> GGUUUCAACAUCCCCG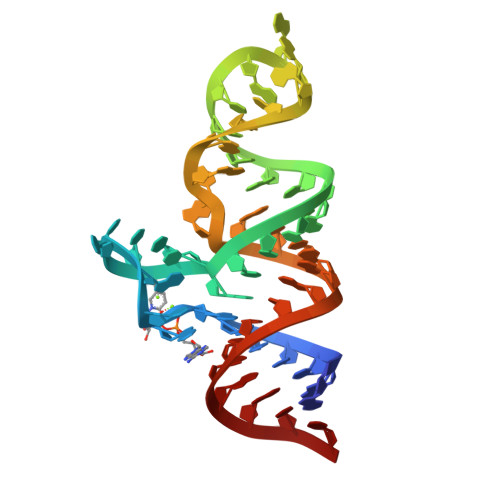UUCGGCGCUCGAAAGAGGUGGCCGGACUGAAGCC>[2x]MSLTLTLTGTGGAQGVPAWGCECAACARARRSPQYRRQPCSGVVKFNDAITLIDAGLHDLADRWSPGSFQQFLLTHYHMDHVQGLFPLRWGVGDPIPVYGPPDEQGCDDLFKHPGLLDFSHTVEPFVVFDLQGLQVTPLPLNHSKLTFGYLLETAHSRVAWLSDTAGLPEKTLKFLRNNQPQVMVMDCSHPPRADAPRNHCDLNTVLALNQVIRSPRVILTHISHQFDAWLMENALPSGFEVGFDGM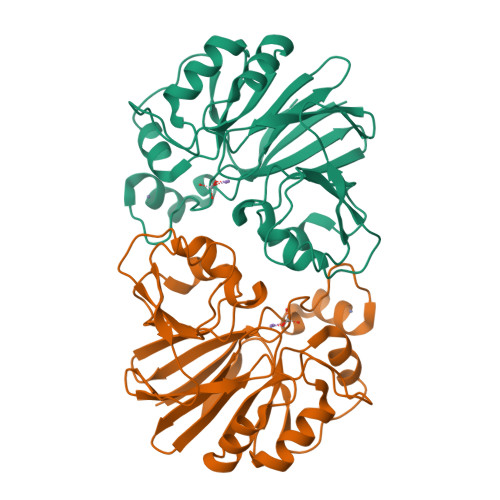EIGVAHHHHHH> GDPMFEARLGQATILKKILDAIKDLLNEATFDCSDSGIQLQAMDNSHVSLVSLTLRSDGFDKFRCDRNLSMGMNLGSMAKI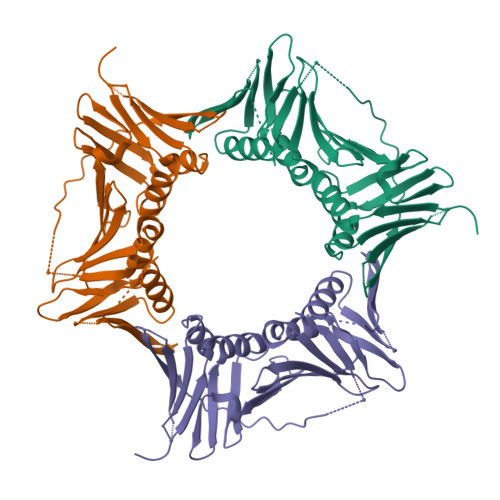LKCANNEDNVTMKAQDNADTVTIMFESANQEKVSDYEMKLMNLDQEHLGIPETDFSCVVRMPAMEFARICRDLAQFSESVVICCTKEGVKFSASGDVGTANIKLAQTGSVDKEEEAVIIEMQEPVTLTFACRYLNAFTKATPLSTQVQLSMCADVPLVVEYAIKDLGHIRYYLAPKIEDNET> GPG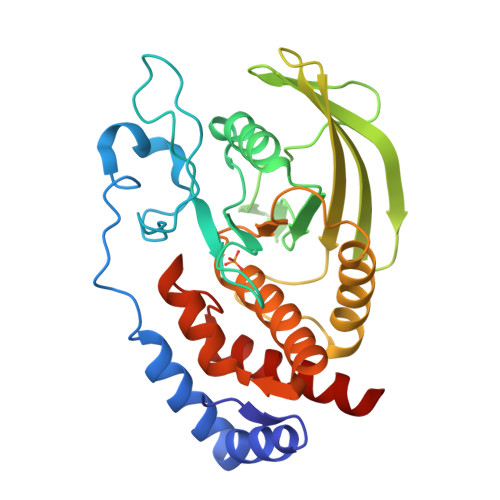DIPAEDFADHVRKNERDSNAGFADEYQQLSLVGHSQSQMVASASENNAKNRYRNVLPYDWSRVPLKPIHEEPGSDYINASFMPGLWSPQEFIATQGPLPQTVGDFWRLVWEQQSHTLVMLTNCMEAGRVKCEHYWPLDSQPCTHGHLRVTLVGEEVMENWTVRELLLLQVEEQKTLSVRQFHYQAWPDHGVPSSPDTLLAFWRMLRQWLDQTMEGGPPIVHSSAGVGRTGTLIALDVLLRQLQSEGLLGPFSFVRKMRESRPLMVQTEAQYVFLHQCILRFLQQSAQA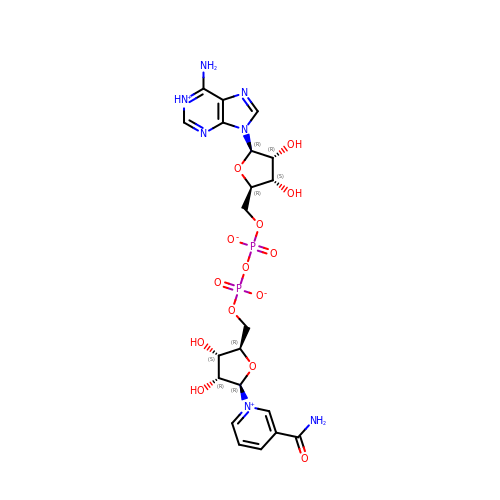NICOTINAMIDE-ADENINE-DINUCLEOTIDE (ACIDIC FORM) | C21 H27 N7 O14 P2 | BAWFJGJZGIEFAR-NNYOXOHSSA-N>MAENTEPRIGVFVCHCGTNIAGSMSIDDVVNYAKTLPYVAVADQYQYMCSTPGQKKIDDAIKEYNLTGVVVAACSPRLHEPTFRTATKEGGLNPFRFEMANIREQNSWVHMHGMWDEATQKAKDQVRMAVAKAAKLEDLVPKSVPVEKTAMVVGGGVAGMQAALDLASAGIKTYLIERTPTIGGRMSQLDKTFPTLDCSQCILTPKMVDVGRHPNIEMMTYTEVEKVEGYIGNFDVTLRKKARGVLTPTEATAKGIVGGGCNGCGDCSAVCPVIKPNPFEMGMAPRKAIYIYHAQVMPLIYTVDFDSCVKCGLCVEACGDKKAIDLEMQDEFITVKVGTAVLATGYELFPIENKREWGYKQFDNVINALEFERLICASGPTGGHLVRPSDGKTPMKVGFVLCAGSRDNTGIGKPYCSRFCCMYSLKHAHQIMEKIPGAVAYLFYMDIRSFGKMYEEFYYRIQHEGAKFIRGRVANVLEDKETKNLHVFTEDTLLGRPVDVEVDLLVLAAAVQPNEGANELRKKFGVSASQDGWMLEAHPKLNPCGTTTAGVFLAGVCQGPKDIPDTVAQAEGAASAASIPIHMGEVELEPYFAMCIDELCAGCGMCVNLCPYSALSLGEKNGRTVMVVTEAKCKGCGTCGGFCPGGAIKMQHFTTPQIVAQIDAFFAGGEQ[2x];>[2x]MHEYAFFLGCIAPNRYPGCEASAIKTSEKVGIKLLPLKGASCCPAPGAFGSIDLNVWYAMAARNLVLAEEMKKDIALICNGCYKSIWEVNHILKHNDELRDNVNEVLAEIDMQFKGTIDVWHLAELYYDDKVCGVQKIKDSVTTPLSGAKVAAHYGCHLMKPKKERHFGDTENPMWFEELIGALGAEPIQYRNKMQCCGAGGGVRGYDIVHALDITNEKLINIQEAGADAITELCPFCQLQFDRGQIEIKEKFGDVYNIPVLHYNELLGLAQGMSPQDLALDLHAIDCTPFLQKVL;>MAAKSYNIPELDKKLADRRYHLSDTNPEFTQKILKTSRTIANMCYQCGTCTGSCPSAPRSSYRIRLFMRRCVLGLENEALTDPDLWLCTTCYSCTDR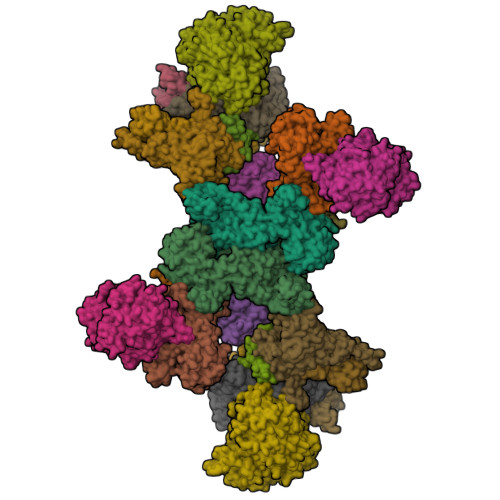CPRDIAPTDVIMAMRNLAFKRDIVPKNFLQTVQLIYNSGHGVPNNDVNRAARTKLGLPADPPTTHSYPEFVKGIQKIIDHYELKENADRILKGD[2x];>[2x]MSENSEIMKYVATTCPYCGVGCTLNLVVSNGKVVGVEPNQRSPINEGKLCPKGVTCWEHIHSPDRLTTPLIKKDGKFIEASWDEALDLVAKNLKVIYDKHGPKGLGFQTSCRTVNEDCYIFQKFARVGFKTNNVDNCARICHGPSVAGLSLSFGSGAATNGFEDALNADLILIWGSNAVEAHPLAGRRIAQAKKKGIQIIAVDPRYTMTARLADTYVRFNPSTHIALANSMMYWIIKEGLEDKKFIQDRVNGFEDLKKTVENYADAEAIHGVPLDVVKDIAFRYAKAKNAVIIYCLGITELTTGTDNVRSMGNLALLTGNVGREGVGVNPLRGQNNVQGACDMGAYPNVYSGYQKCEVAENRAKMEKAWSVTNLPDWYGATLTEQINQCGDEIKGMYILGLNPVVTYPSSNHVKAQLEKLDFLVVQDIFFTETCQYADVILPGACFAEKDGTFTSGERRINRVRKAVNPPGQAKEDIHIISELAAKMGFKGFELPTAKDVWDDMRAVTPSMFGATYEKLERPEGICWPCPTEEHPGTPILHREKFATADGKGNLFGIDYRPPAEVADAEYPFTLMTGRLIFHYHSRTQTDRAADLHREVPESYAQINIEDARRLGIKNNEYIKLKSRRGETTTLARVTDEVAPGVVYMTMHFADGVNNLTNTVLDPMSKMPELKHCAISIEKVGGN;>MAAKGDMLYAWAKDAEIQKKGECGGAVTALLKHALETKMVDAVVAIKKGKDLYDAVPTVITNPEDIIQTAGSLHCGTLLIPKLIKKYLNGAKDMKLAVTCKGCDAMAFYELAKRNQINLDNIIMIGVNCGGSVSPVTARKMISNKFGVDPDTVHKEEIDKGQFIIEYEGGHKGIKIDELEEEGYGRRSNCRRCKMKIPRQADIAAGNWGVIGDKAGKATFLEICSEKGANLVNSAQSKGALEISPADPKGIDIRAKVEKAMFNLGDEWRHRDFEGMGKGKDRLKLMMSESSKCIKCYACVEACPICYCIECSTKKPWYIAPGVLPTSFMFHLIRFAHVSDSCINCGQCEELCPMEIPNALFMHSQQVEIEKMFGHIPGQDMTPPIHAFVEEKAERARLDATGTDSIYTNIFTDE[2x];>[2x]MADDWKPQILAIICNWCSYAGADLAGGARIQYPPTVRAIRVMCTGRVDMLFILKAFVEGADGVLVSGCHFGDCHYLEGNYKAAKRMFMIKNLLRNIGLDDRRFRMTFVSASEGAKWGMVMEDVTNTIKELGPSPIKEFKK;>MSELLIKNGYIFDPISGIKGDKADIAIKDGKIVDKVSSKAQVIDASGKTVMSGGVDIHTHVSGPKVNTGRMMRPEDKFFRGSYRGGIIKQGKRMEMGFSIPSTYKTGYAYARMGYTFTNEAAMPPLLAPHVHEEFRDTPILDQAAMPVFGNNWFCFEYIKNKELENNAAYVAWLLNATKGIGIKVVNPGGTEAWAWGENCTTINDPVPYFDITPAEIVKGLIETNEYLGLPHSVHIHGNNLGNPGNYKDTLDTLRLAESYKAKNKFGREQVLHNTHIQFHSYKGTSWADFESGAKEIMDYVNANKNITCDIGQVTLDETTTMTADGPFEYHLNQLNHIKWANVDVELETGSGVVPYIYDKNIKVCGIQWAIGLELALYAKDLMRVHITTDHPNAGPFTRYPCVIKWLMSEKARKATLDTMKWKDKVIAASNIASMDRELGLYEIAMMTRAGPAKALGLAAIYGSLVKGADGNVAIYNLDANDLPSDPELIEAAFQNTAYTIKEGVVVVKDGEIIAEPHKYTLWTKVNMPENAQVMHDIKEKFTKNYTVNLENYAVFDEHVHNPRAIELDVA[2x];>MPKVIENVGCPYCGCSCDDVRITVSDDGKDILEVENVCAIGTEIFKHGCSKDRIRLPRMRQPDGSMKDISYEEAIDWTARHLLKAKKPLMYGFGSTNCEGQAAAARVMEIAGGMLDNCATICHGPSFLAIFDNGYPSCTLGEVKNRADVIVYWGSNPAHAHPRHMSRYSIFPRGFFTGKGQKKRTVIVIDPRFTDTANVADYHLQVKQGHDYELFNAFRMVIHGHGKDLPDEVAGIKKETILEVAEIMKNARFGTTFFGMGLTHTDGRNHNIDIAISLTRDLNKISKWTIMAMRGHYNIAGPGVVWSWTFGFPYCLDLTKQNHAHMNPGETSSVDMAMRDEVDMFINIGTDAAAHFPIPAVKQLKKHPWVTIDPSINMASEISDLHIPVCICGVDVGGIVYRMDNVPIQFRKVIEPPEGVMDDETLLNKIADRMEELKAKGEA[2x];>METITMTLVQEPELFLECYSVTPDLFAGKSLAEIADLPAHEGKIQWKLGDFFKFEGKAGETAADTKIVVNGNVRRMKRFGQQMTAGEIIINSDADMYIGGWMKGGKITVKGNADSFLGIAMEGGEILIEGDAQNHVGSAYRGDWRGMSGGLIRVKGKAGNDIGTAMTGGTIIIEGDAFIHVLTHAEGGTVIIKGDVEGRVGGQMVKGDAYILGNLLYPLPGFKKVATVEKEVDGATYTFDQFIGDLGERKEKKKGEIIYGNIFLKK[2x];>MKAKKTLNMITQRAVEEGIAMEIGKTSRQYFDACSIIEMNEQDMKELGIMKNTNVRVKSESGEVVVKAVVGRQTCYPGLCHIRQGVWANQVVPPRTQSTGAPQYSGFPVTVEPVPNERLKTALELVQGAVGMWKGDQ[2x];>MSTLFPKYSKTTDGSKVIMEQRLLQQVNNLILDNDICTGCGICSEVCPEEAISVGAVGGVRRGLVDDAASIHVDETKCSYCGVCVIMCPFSALALKVDGEERLPILEKEGFPTYDKGTAIDQDKCVRCNICDDVCPRDAIDRDVPLFEGEDKEGLAKGQAVELKIEFKVDDEKCTKCGICGNLCEAINVLHKPFSPEIGKVEGEVIWDEAYCDGCNVCAEACPSEAIKVTRTVVGQKKLGNVNIIDEDCCTCRWCAINCPTEAITVNKIFEGEITFHAEKCPGGCSTCVDVCPANAIYLPTPKPAKDMKGQIEAKIAVNKDFCILCGACVNACPGEDIIYLRRDSVKIKGKETDLFKKIKEKLFTPRTSKVKEQPSLAGSVELKAVSQ[4x];>[2x]MKYRGPEDKLIVFTFYKESKKKRHFFPFFLQKISYLFQNIYLYFLTTFVQSILIDQAGATNMAFAVHVNMERCTGCNNCVVACPVNALELNTVNPSSTDKIYKVINGDAVILDVKHELCAGCGICVDACPYDVIQLSGQPPQAVEA>[4x]MTPILAAEALTYAFPGGVKALDDLSLAVPKGESLAILGPNGAGKSTLLLHLNGTLRPQSGRVLLGGTATGHSRKDLTGWRRRVGLVLQDADDQLFATTVFEDVSFGPLNLGLSEAEARARVEEALAALSISDLRDRPTHMLSGGQKRRVAIAGAVAMRPEVLLLDEPTAGLDLAGTEQLLTLLRGLRAAGMTLVFSTHDVELAAALADRVALFRTGRVLAEGAAEAVLSDRATLAKVALRPPLVIDLALLARDHGLLAPEAPLPKTRDALAAQMAGWTRR;>[2x]MHIMEGYLPVTHAIGWSLAAAPFVVAGALKIRKIVAERPEARMTLAAAGAFAFVLSALKIPSVTGSCSHPTGTGLGAVVFGPSVMAVLGVIVLLFQALLLAHGGLTTLGANAFSMAIVGPWVAFGVYKLAGKAGASMAVAVFLAAFLGDLATYVTTSLQLALAYPDPASGFLGAALKFGSVFALTQIPLAIAEGFLTV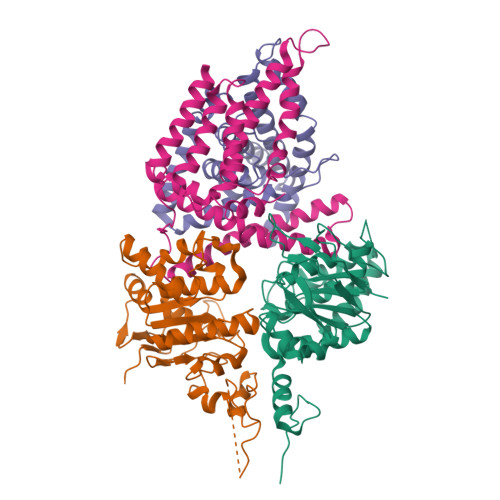IVVDALAGKVADEDKLRILAGEAR;>MGSHHHHHHSGSMSIASIDRVAAQGHWRSRPLAEKSLIGLGFLALAVTVPPFPGAVLVTVAILAFTFLGARVPLRFWASVAVLPLGFLTTGAAVLLIQIGPEGIGLAPDGPAKAAALVMRATAATCCLLFLATTTPAADLLSGLRRWRVPAELIEIALLTYRFVFILAEEAAAMTTAQRARLGHATRRRWLRSTAQVIAALLPRALTRARRLETGLGARNWQGEMRVLSTRPPASARVLGLILTLQAAILAAGVLL[2x]>MSIFPKISLRPEVENYLKEGFMNKEIVTALGKQEAERKFETLLKHLSHPPSFTTVRVNTHLASVQHVKNLLLDELQKQFNGLSVPILQHPDLQDVLLIPVIGPRKNIKKQQCEAIVGAQCGNAVLRGAHVYAPGIVSASQFMKAGDVISVYSDIKGKCKKGAKEFDGTKVFLGNGISELSRKEIFSGLPELKGMGIRMTEPVYLSPSFDSVLPRYLFLQNLPSALVSHVLNPQPGEKILDLCAAPGGKTTHIAALMHDQGEVIALDKIFNKVEKIKQNALLLGLNSIRAFCFDGTKAVKLDMVEDTEGEPPFLPESFDRILLDAPCSGMGQR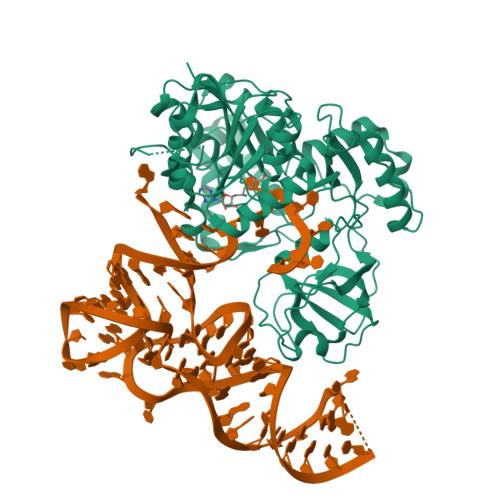PNMACTWSVKEVASYQPLQRKLFTAAVQLLKPEGVLVYSTCTITLAENEEQVAWALTKFPCLQLQPQEPQIGGEGMRGAGLSCEQLKQLQRFDPSAVPLPDTDMDSLREARREDMLRLANKDSIGFFIAKFVKCKSTLEHHHHHH[2x]>NLIPTVIEQTNRGERAYDIYSRLLKDRIIMLGSAIDDNVANSIVSQLLFLAAEDPEKEISLYINSPGGSITAGMAIYDTMQFIKPKVSTICIGMAASMGAFLLAAGEKGKRYALPNSEVMIHQPLGGAQGQATEIEIAAKRILLLRDKLNKVLAERTGQPLEVIERDTDRD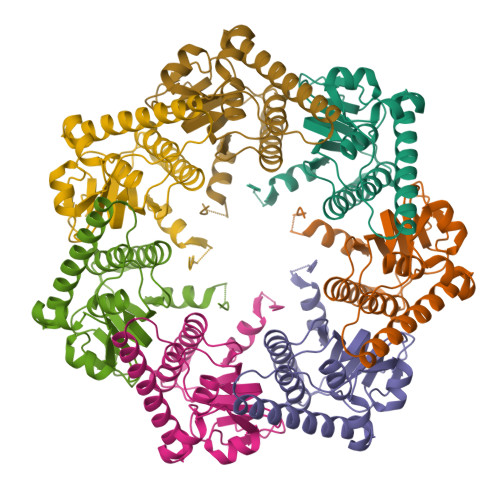NFKSAEEALEYGLIDKILTHLEHHHHHH[7x]> PISPIETVPVKLKPGMDGPKVKQWPLTEEKIKALVEICTELEKEGKISKIGPENPYNTPVFAIKKKDSTKWRKLVDFRELNKRTQDFWEVQLGIPHPAGLKKKKSVTVLDVGDAYFSVPLDEDFRKYTAFTIPSINNETPGIRYQYNVLPQGWKGSPAIFQSSMTKILEPFRKQNPDIVIYQYMDDLYVGSDLEIGQHRTKIEELRQHLLRWGLYTPDKKHQKEPPFLWMGYELHPDKWTVQPIVLPEKDSWTVNDIQKLVGKLNWASQIYPGIKVRQLCKLLRGTKALTEVIPLTEEAELELAENREILKEPVHGVYYDPSKDLIAEIQKQGQGQWTYQIYQEPFKNLKTGKYARMRGAHTNDVKQLTEAVQKITTESIVIWGKTPKFKLPIQKETWETWWTEYWQATWIPEWEFVNTPPLVKLWYQLEKEPIVGAETFYVDGAANRETKLGKAGYVTNRGRQKVVTLTDTTNQKTELQAIYLALQDSGLEVNIVTDSQYALGIIQAQPDQSESELVNQIIEQLIKKEKVYLAWVPAHKGIGGNEQVDKLVSAGIRKVL;> PISPIETVPVKLKPGMDGPKVKQWPLTEEKIKALVEICTELEKEGKISKIGPENPYNTPVFAIKKKDSTKWRKLVDFRELNKRTQDFWEVQLGIPHPAGLKKKKSVTVLDVGDAYFSVPLDEDFRKYTAFTIPSINNETPGIRYQYNVLPQGWKGSPAIFQSSMTKILEPFRKQNPDIVIYQYMDDLYVGSDLEIGQHRTKIEELRQHLLRWGLYTPDKKHQKEPPFLWMGYELHPDKWTVQPIVLPEKDSWTVNDIQKLVGKLNWASQIYPGIKVRQLCKLLRGTKALTEVIPLTEEAELELAENREILKEPVHGVYYDPSKDLIAEIQKQGQGQWTYQIYQEPFKNLKTGKY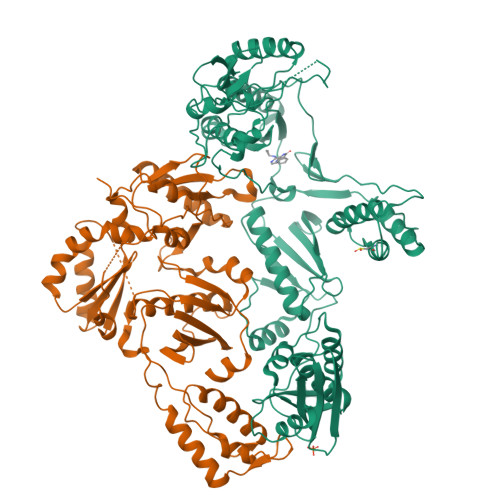ARMRGAHTNDVKQLTEAVQKITTESIVIWGKTPKFKLPIQKETWETWWTEYWQATWIPEWEFVNTPPLVKLWYQLEKEPIVGAETF> SIPWNLERITPPRYRADEYQPPDGGSLVEVYLLDTSIQSDHREIEGRVMVTDFENVPEEDGTRFHRQASKCDSHGTHLAGVVSGRDAGVAKGASMRSLRVLNCQGKGTVSGTLIGLEFIRKSQLVQPVGPLVVLLPLAGGYSRVLNAACQRLARAGVVLVTAAGNFRDDACLYSPASAPEVITVGATNAQDQPVTLGTLGTNFGRCVDLFAPGEDIIGASSDCSTCFVSQSGTSQAAAHVAGIAAMMLSAEPELTLAELRQRLIHFSAKDVINEAWFPEDQRVLTPNLVAALPPSTHGAGWQLFCRTVWSAHSGPTRMATAVARCAPDEELLSCSSFSRSGKRRGERMEAQGGKLVCRAHNAFGGEGVYAIA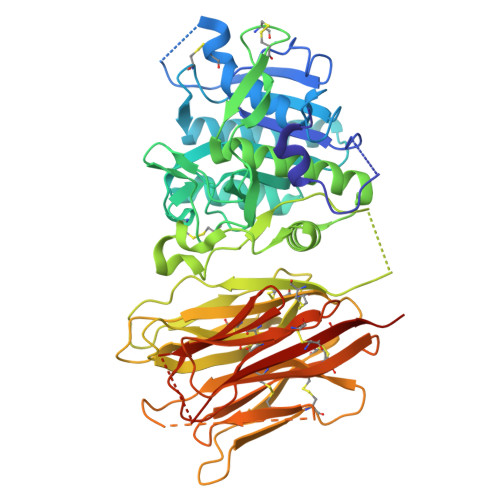RCCLLPQANCSVHTAPPAEASMGTRVHCHQQGHVLTGCSSHWEVEDLGTHKPPVLRPRGQPNQCVGHREASIHASCCHAPGLECKVKEHGIPAPQEQVTVACEEGWTLTGCSALPGTSHVLGAYAVDNTCVVRSRDVSTTGSTSEGAVTAVAICCRSRHLAQASQELQ> MVFKKVLLTGTSEESFTAAADDAIDRAEDTLDNVVWAE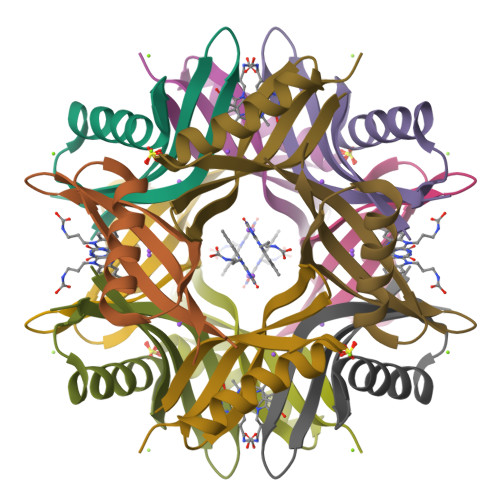VVDQGVAIGAVRTYQTEVQVAFELDGSQLEHHHHHH>[2x]MELWLVRHGETLWNREGRLLGWTDLPLTAEGEAQARRLKGALPSLPAFSSDLLRARRTAELAGFSPRLYPELREIHFGALEGAMWETLDPRYKEALLRFQGF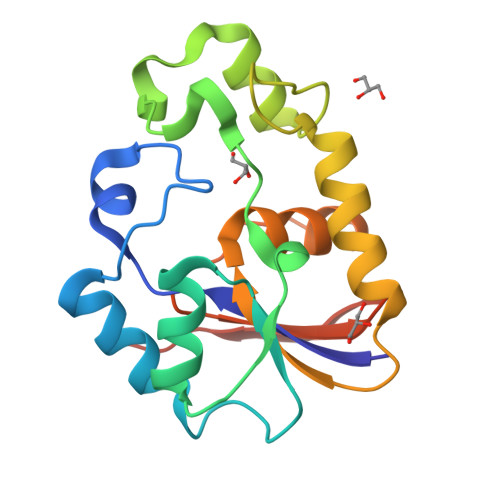HPPGGESLSAFQERVFRFLEGLKAPAVLFTHGGVVRAVLRALGEDGLVPPGSAVAVDWPRRVLVRLALDGEEATG>GPGTMDVTFLTKNVQINGTQFKILLQNGQGECALIALANVLLISPAHARYAQEISRLVRGKETVTLNELVQTLADMGVQNPNGTDVDKQQLLQILPQLYSGLNINPEFNGSFEDGVEMSIFRLYNVGIVHGWIID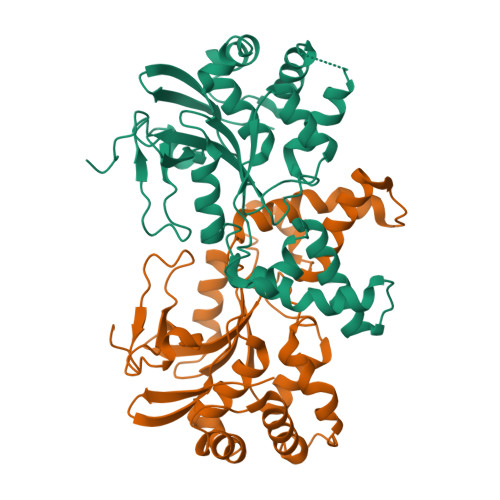GDNDPNSYEHVSKYSYMGAQKVLVQSYEIQKNNAQFENSEQIQSDAPYLKSFLARSATQLTEYGLTHLREILVERSYAVLFRNDHFCTLYKNNGELFTLVTDPTYRNRKDINWQSLKSVNGSQDSYYTGNFIPTSLERTETTATGQNE[2x]>[2x]MKKRLTITLSESVLENLEKMAREMG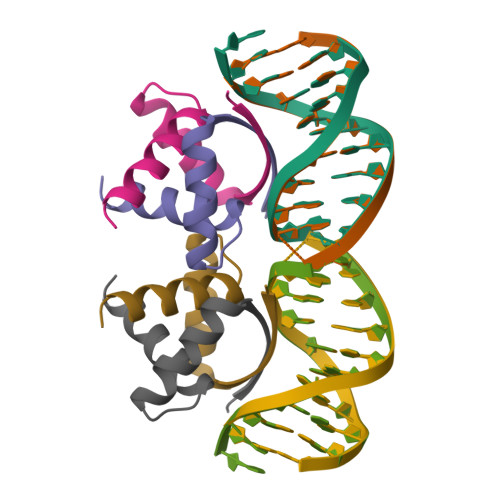LSKSAMISVALENYKKGQEK> ISPIETVPVKLKPGMDGPKVKQWPLTEEKIKALVEICTEMEKEGKISKIGPENPYNTPVFAIKKKDSTKWRKLVDFRELNKRTQDFWEVQLGIPHPAGLKKKKSVTVLDVGDAYFSVPLDEDFRKYTAFTIPSINNETPGIRYQYNVLPQGWKGSPAIFQSSMTKILEPFRKQNPDIVIYQYMDDLCVGSDLEIGQHRTKIEELRQHLLRWGLTTPDKKHQKEPPFLWMGYELHPDKWTVQPIVLPEKDSWTVNDIQKLVGKLNWASQIYPGIKVRQLCKLLRGTKALTEVIPLTEEAELELAENREILKEPVHGVYYDPSKDLIAEIQKQGQGQWTYQIYQEPFKNLKTGKYARMRGAHTND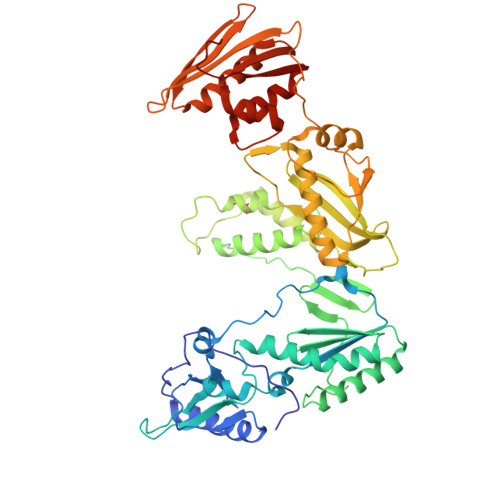VKQLTEAVQKITTESIVIWGKTPKFKLPIQKETWETWWTEYWQATWIPEWEFVNTPPLVKLWYQLEKEPIVGAETFYVDGAANRETKLGKAGYVTNRGRQKVVTLTDTTNQKTELQAIYLALQDSGLEVNIVTDSQYALGIIQAQPDQSESELVNQIIEQLIKKEKVYLAWVPAHKGIG> SMADLIAIITPAHDNPFFKAEAVGAEAKAKELGYETLVMTHDDD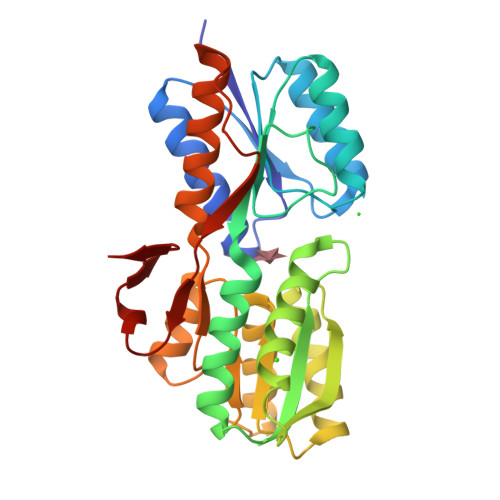ANKQSEMIDTAIGRGAKAIILDNAGADASVAAVKKAKDAGIPSFLIDREINATGVAVAQIVSNNYQGAQLGAQEFVKLMGEKGNYVELVGKESDTNAGIRSQGYHDVIDDYPEMKSVAKQSANWSQTEAYSKMETILQANPDIKGVISGNDTMAMGAIAALQAAGRKDVIVVGFDGSNDVRDSIKSGGIKATVLQPAYAQAQLAVEQADAYIKNKTTPKEEKQLMDCVLINADNAGKLETFALTN>[11x]MIKRVLVVSMVGLSLVGCVNNDTL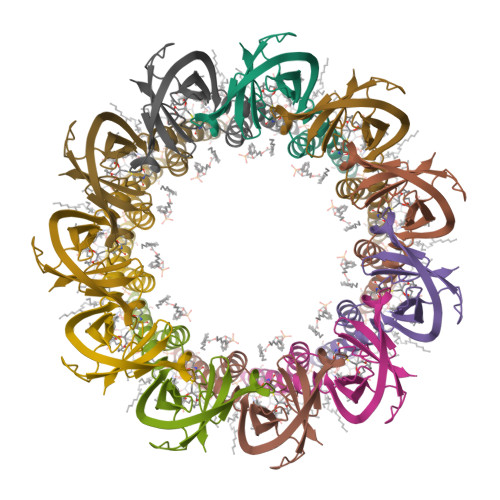SGDVYTASEAKQVQNVSYGTIVNVRPVQIQGGDDSNVIGAIGGAVLGGFLGNTVGGGTGRSLATAAGAVAGGVAGQGVQSAMNKTQGVELEIRKDDGNTIMVVQKQGNTRFSPGQRVVLASNGSQVTVSPR>MHHHHHHSTNELDVNDIYDHLNEKYSQFNDVTFSKPSTNYLKPGWILDTHFTFGTSSEFYNKSFDALSFNHVDSEFNMSTCNDDSECGGVSTCTAPAYTKNKDGDAKKLCTVPADKILDAIYDNIVSAKRSVDIVTLQPMDISHLNLSFSSGAFTATIKNALSQLAKNTQYSDHHI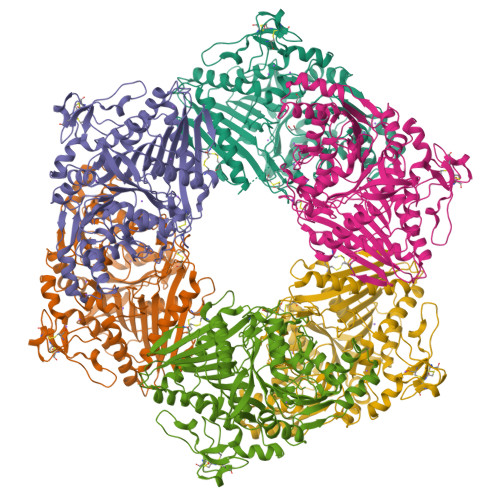TVRLLQGSFTPMLGYDAESEEEEIRQLSLTQTNYLSEIASVLPEVNNLDITVGSVRSCNKLISNCGNNNSQKDVLLNVAWNHGKIINVDNQSVITGGHNLWGADYLQRNPVNDLSINILGPIASTATKYGNTLWNYVCNNTGTITNTFVTYANGQYTYDCPAHISSTYVAPTDAKNGLAVKVMSISKLNNGVLDKDADQSEVARVYAFKNATKSIKISQQALFFKGAFGKVLHPLKTIDGTVMEALASAIYKGVTVDIVTSSLDGGIYSSGYNSEFVYNYLLNVLHKAPYYLERNYAKTFLDKNLHINFISINGRETNNMSHNKLWIVDDKVFYVGSHNIYPSSLQQFGVIVDDKDATAQLEKQLWTPMWKNSIHVPINNS[6x]>MASVQLQNVTKAWGEVVVSKDINLDIHEGEFVVFVGPSGCGKSTLLRMIAGLETITSGDLFIGEKRMNDTPPAERGVGMVFQSYALYPHLSVAENMSFGLKLAGAKKEVINQRVNQVAEVLQLAHLLDRKPKALSGGQRQRVAIGRTLVAEPSVFLLDEPLSNLDAALRVQMRIEISRLHKRLGRTMIYVTHDQVEAMTLADKIVVLDAGRVAQVGKPLELYHYPADRFVAGFIGSPKMNFLPVKVTATAIDQVQVELPMPNRQQVWLPVESRDVQVGANMSLGIRPEHLLPSDIADVILEGEVQVVEQLGNETQIHIQIPSIRQNLVYRQNDVVLVEEGATFAIGLPPERCHLFREDGTACR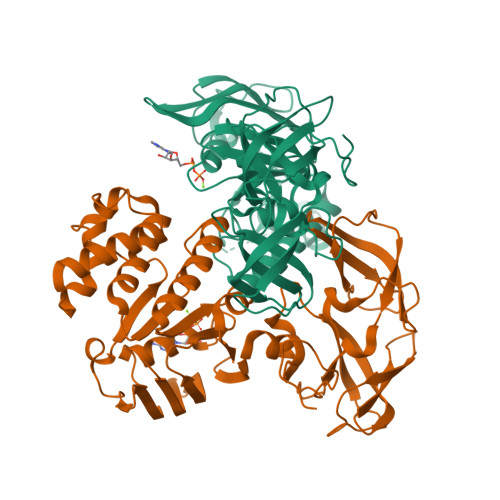RLHKEPGVASASHHHHHH[4x]>GGAGCUCGCCC[2x];>[2x]GGGCGAGGCCGUGCCGGC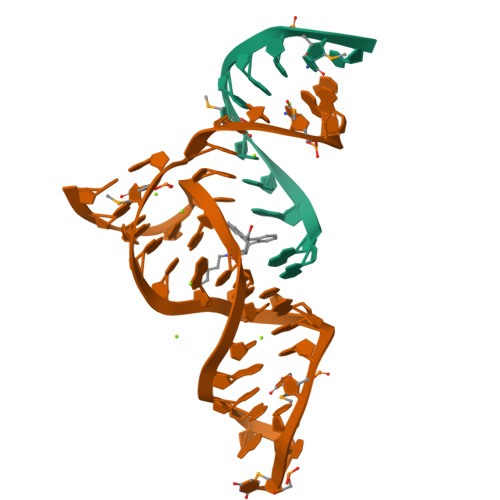UCUUCGGAGCAAUACUCGGC>SNAKPITVMLLGSGESGKSTIAKQLKILFGGGFPEQERATHKSSICSNVVTCMRTLIEQSAILNHPMKYQPKSKEFTTEDPVTLPFSPELVGDVEALWADEGIQATYEESAKFQLPDCAKYLFENVKRIAMEDYVPTEEDLIHNRTKTTGIHEYDFVVKDIPFHLIDVGGQRSERKKWVSFFSDVDCAIFVTSLAEYDMKLYEDGNTSRLTESIAVFKDIMTNEFLKGAVKLIFLNKMDLFEEKLTKVPLNTIFPEYTGGDNAVMGAQ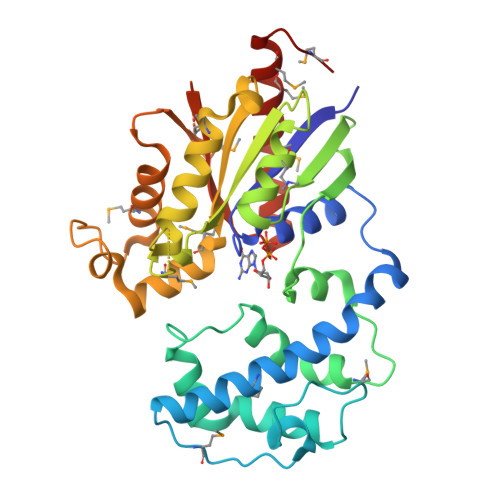YIQQLFTGKLQTEEMNISGADGTANIEGAVNEKVYTNPTNATDGSNIKRVFMLAVDVIMKNMAANGKMRPTK[2x]> EMAKPVLPDLSGYTTEAALKKIARNKPGKITVARMMEETGLKEFIGGDNKMAEWVVRQKGIPQAIMISDGYVNLQDLVKKVPKQFLSEVSPGVYVARLPILVKETGIFEIDSKTKELRLSQEKGSFIVSEGKMLITNTSVNAWSETRNGLAAYRTPDEFRPFVLTWGGSQTWIAKTKMASMGYNQSKSYGVSISQYNPNMAKVLKRGEPTGWIIDSEFADMWYGFYCYETRDFVVKGNTYRDNIVYGIDPHDRSHGLIIAENDVYGTKKKHGIIISREVDNSFIFRNKSHNNKLSGVVLDRNSVGNIVAYNEIYQNHTDGITLYESGNNLLWGNRVIANRRHGIRVRNSVNIKLYENVAMANGLMGVYGHIKDLNDTDRDIELDPFDAQVSLIMVGGELSSNGSGPLSIDSPLSV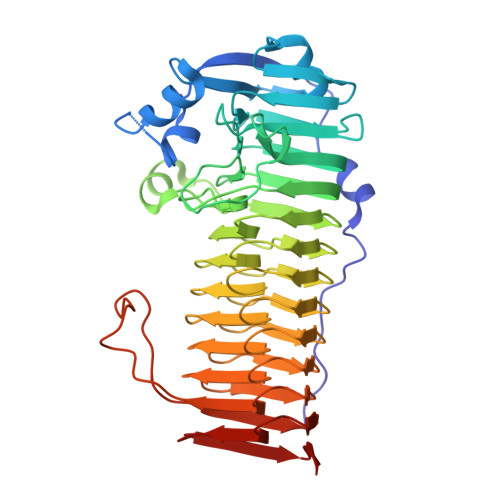ELYRVSMLM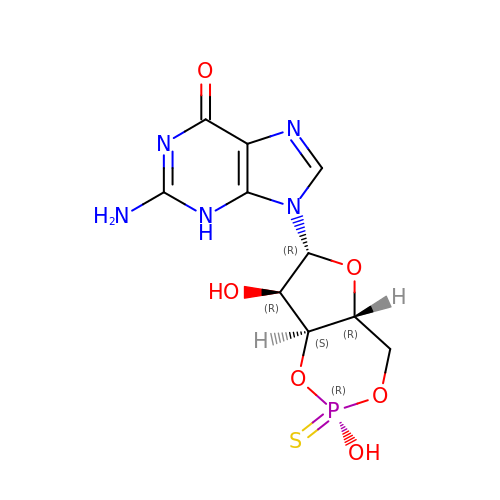2-amino-9-[(2R,4aR,6R,7R,7aS)-2,7-dihydroxy-2-sulfanylidenetetrahydro-2H,4H-2lambda~5~-furo[3,2-d][1,3,2]dioxaphosphinin-6-yl]-3,9-dihydro-6H-purin-6-one | C10 H12 N5 O6 P S | JZAJZXRXCHCRMU-KVBUDSETSA-N>MPGEIRPTIGQQMETGDQRFGDLVFRQLAPNVWQHTSYLDMPGFGAVASNGLIVRDGGRVLVVDTAWTDDQTAQILNWIKQEINLPVALAVVTHAHQDKMGGMDALHAAGIATYANALSNQLAPQEGMVAAQHSLTFAANGWVEPATAPNFGPLKVFYPGPG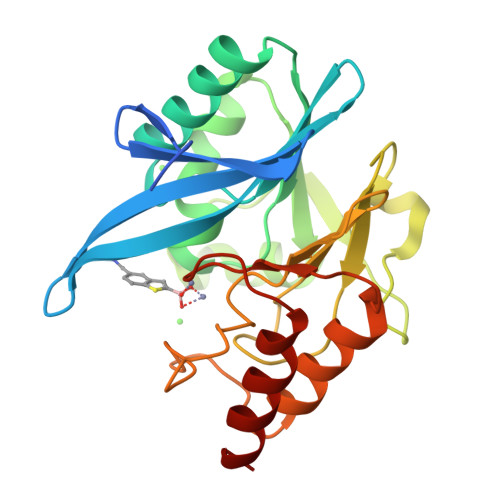HTSDNITVGIDGTDIAFGGCLIKDSKAKSLGNLGDADTEHYAASARAFGAAFPKASMIVMSHSAPDSRAAITHTARMADKLR[2x]>[4x]MGSSHHHHHHSSGLVPRGSHMSRFVQDLSKAMSQDGASQFQEVIRQELELSVKKELEKILTTASSHEFEHTKKDLDGFRKLFHRFLQEKGPSVDWGKIQRPPEDSIQPYEKIKARGLPDNISSVLNKLVVVKLNGGLGTSMGCKGPKSLIGVRNENTFLDLTVQQIEHLNKTYNTDVPLVLMNSFNTDEDTKKILQKYNHCRVKIYTFNQSRYPRINKESLLPVAKDVSYSGENTEAWYPPGHGDIYASFYNSG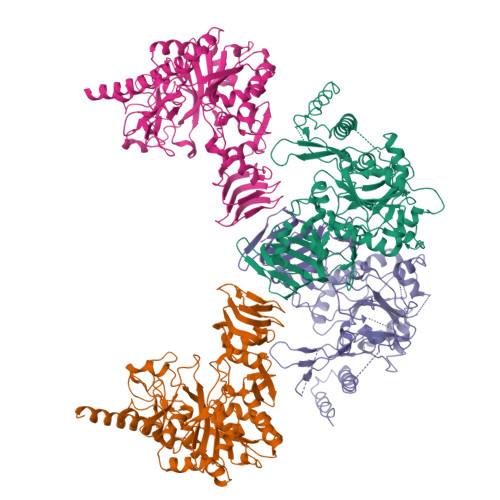LLDTFIGEGKEYIFVSNIDNLGATVDLYILNHLMNPPNGKRCEFVMEVTNKTRADVKGGTLTQYEGKLRLVEIAQVPKAHVDEFKSVSKFKIFNTNNLWISLAAVKRLQEQNAIDMEIIVNAKTLDGGLNVIQLETAVGAAIKSFENSLGINVPRSRFLPVKTTSDLLLVMSNLYSLNAGSLTMSEKREFPTVPLVKLGSSFTKVQDYLRRFESIPDMLELDHLTVSGDVTFGKNVSLKGTVIIIANHGDRIDIPPGAVLENKIVSGNLRILDH>[2x]SGDY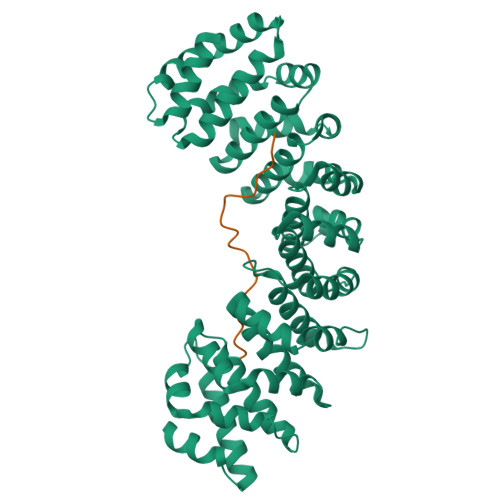RVQNTSLEAIVQNASSDNQGIQLSAVQAARKLLSSDRNPPIDDLIKSGILPILVHCLERDDNPSLQFEAAWALTNIASGTSEQTQAVVQSNAVPLFLRLLHSPHQNVCEQAVWALGNIIGDGPQCRDYVISLGVVKPLLSFISPSIPITFLRNVTWVMVNLCRHKDPPPPMETIQEILPALCVLIHHTDVNILVDTVWALSYLTDAGNEQIQMVIDSGIVPHLVPLLSHQEVKVQTAALRAVGNIVTGTDEQTQVVLNCDALSHFPALLTHPKEKINKEAVWFLSNITAGNQQQVQAVIDANLVPMIIHLLDKGDFGTQKEAAWAISNLTISGRKDQVAYLIQQNVIPPFCNLLTVKDAQVVQVVLDGLSNILKMAEDEAETIGNLIEECGGLEKIEQLQNHENEDIYKLAYEIIDQFFSSDDIDEDPSLVPEAIQGGTFGFNSSANVPTEGFQF;>SRRRRRRKRKREWDDDDDPPKKRRRLD[2x]>[4x]GPHMRPLKQA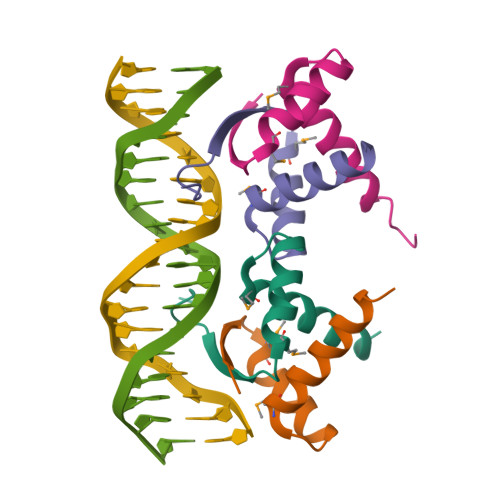TPTYSSRTADKFVVRLPEGMREQIAEVARSHHRSMNSEIIARLEQSLLQEGALQDNLGV>MAASATAAAVAAEVISVHSLEQWTMQIEEANTAKKLVVIDFTASWCGPCRIMAPVFADLAKKFPNAVFLKVDVDELKPIAEQFSVEAMPTFLFMKE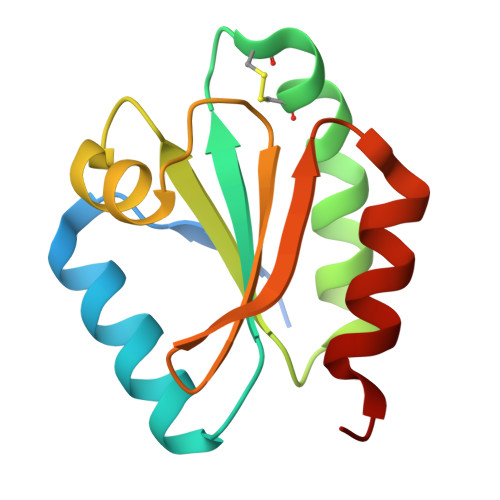GDVKDRVVGAIKEELTAKVGLHAAAQ[2x]>[2x]AELVSDKALESAPTVGWASQNGFTTGGAAATSDNIYIVTNISEFTSALSAGAEAKIIQIKGTIDISGGTPYTDFA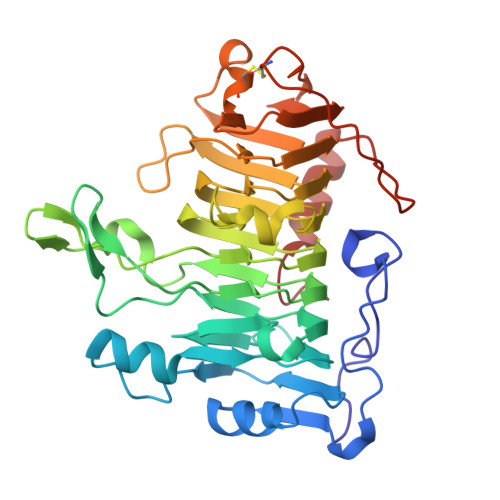DQKARSQINIPANTTVIGLGTDAKFINGSLIIDGTDGTNNVIIRNVYIQTPIDVEPHYEKGDGWNAEWDAMNITNGAHHVWIDHVTISDGNFTDDMYTTKDGETYVQHDGALDIKRGSDYVTISNSLIDQHDKTMLIGHSDSNGSQDKGKLHVTLFNNVFNRVTERAPRVRYGSIHSFNNVFKGDAKDPVYRYQYSFGIGTSGSVLSEGNSFTIANLSASKACKVVKKFNGSIFSDNGSVLNGSAVDLSGCGFSAYTSKIPYIYDVQPMTTELAQSITDNAGSGKL>[2x]STKVVNVAVIGAGVVGSAFLDQLLAMKSTITYNLVLLAEAERSLISKDFSPLNVGSDWKAALAASTTKTLPLDDLIAHLKTSPKPVILVDNTSSAYIAGFYTKFVENGISIATPNKKAFSSDLATWKALFSNKPTNGFVYHEATVGAGLPIISFLREIIQTGDEVEKIEGIFSGTLSYIFNEFSTSQANDVKFSDVVKVAKKLGYTEPDPRDDLNGLDVARKVTIVGRISGVEVESPTSFPVQSLIPK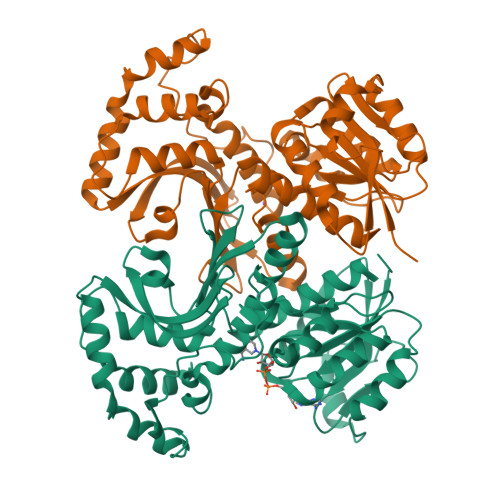PLESVKSADEFLEKLSDYDKDLTQLKKEAATENKVLRFIGKVDVATKSVSVGIEKYDYSHPFASLKGSDNVISIKTKRYTNPVVIQGAGAGAAVTAAGVLGDVIKIAQRL> GSDEKRLHFGNGHLKLPGLRTFVDPHTFEDPTQTVHEFAKELDATNISIDKVVGAGEFGEVCSGRLKLPSKKEISVAIKTLKVGYTEKQRRDFLGEASIMGQFDHPNIIRLEGVVTKSKPVMIVTEYMENGS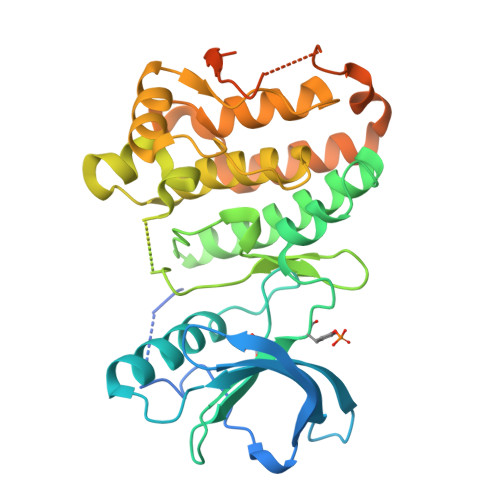LDSFLRKHDAQFTVIQLVGMLRGIASGMKYLSDMGAVHRDLAARNILINSNLVCKVSDFGLSRVLEDDPEAAYTTRGGKIPIRWTSPEAIAYRKFTSASDVWSYGIVLWEVMSYGERPYWEMSNQDVIKAVDEGYRLPPPMDCPAALYQLMLDCWQKDRNNRPKFEQIVSILDKLIRNPGSLKIITSAAARPSNLLLDQSNVDITTFRTTGDWLNGVWTAHCKEIFTGVEYSSCDTIAKIS>GSHMKIRQRFRFGRLELKRISGRGFKNDEEILIGNGTIQKIGIWDGEEEFHVRCGECRGILKKSKMKLEKLLINSAKKEDMRDLIILCMVFSQDTRMFQGVRGEINFLNRAGQLLSPMYQLQRYFLNRSSDLFDQWGYEESPKASELHGINES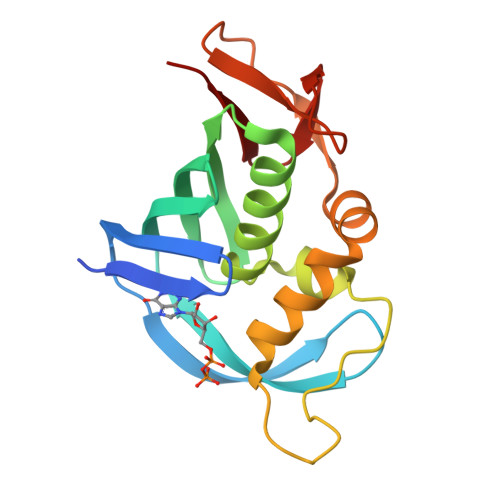MNASDYTLKGVVVTKN[2x]> PISPIETVPVKLKPGMDGPKVKQWPLTEEKIKALVEICTEMEKEGKISKIGPENPYNTPVFAIKKKDSTKWRKLVDFRELNKRTQDFWEVQLGIPHPAGLKKKKSVTVLDVGDAYFSVPLDEDFRKYTAFTIPSINNETPGIRYQYNVLPQGWKGSPAIFQSSMTKILEPFRKQNPDIVIYQYMDDLYVGSDLEIGQHRTKIEELRQHLLRWGLTTP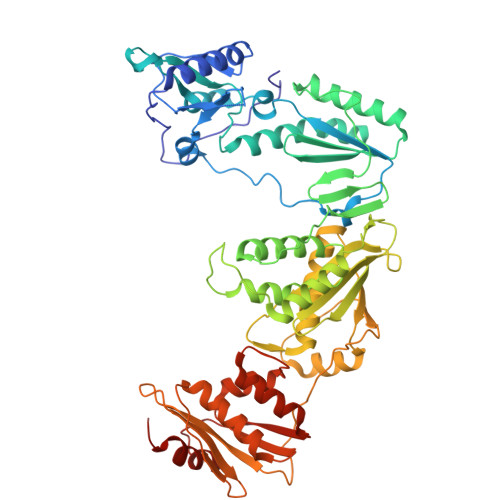DKKHQKEPPFLWMGYELHPDKWTVQPIVLPEKDSWTVNDIQKLVGKLNWASQIYPGIKVRQLCKLLRGTKALTEVIPLTEEAELELAENREILKEPVHGVYYDPSKDLIAEIQKQGQGQWTYQIYQEPFKNLKTGKYARMRGAHTNDVKQLTEAVQKITTESIVIWGKTPKFKLPIQKETWETWWTEYWQATWIPEWEFVNTPPLVKLWYQLEKEPIVGAETFYVDGAANRETKLGKAGYVTNRGRQKVVTLTDTTNQKTELQAIYLALQDSGLEVNIVTDSQYALGIIQAQPDQSESELVNQIIEQLIKKEKVYLAWVPAHKGIGGNEQVDKLVSAGIRKVLF> SNAPRRSIHLSNIVEQRVFEDDEIISTPKRGRSKKTVQDNDEDYSPKKSVQKTPTRTRRSSTTTKTATTPSKGITTATATPMTPSQKMKKIRAGELSPSMQQRTDLPAKDSSKSELQLAREQLHVSVVPKSLPCREREFENIYAFLEGKIQDQCGGCMYVSGVPGTGKTATVTGVIRTLQRMAKQNELPAFEYLEINGMRLTEPRQAYVQIYKQLTGKTVSWEQAHALLEKRFTTPAPRRVTTVLLVDELDILCNRRQDVVYNLLDWPTKSAAKLVVVTIANTMDLPERLLMGKVTSRLGLTRLTFQPYSHKQLQEIVTARLGGSETFKGEAVQLVARKVAAVSGDARRALDICRRATEIADTAAVKCVTMLHVQQALAEMIASAKVQAIRNCSRMEQIFLQAIAAEVTRTGVEETTFMGVYQQVETIAAFMGVTFPPPGRALRLCSKLGAERLIISEHSRNDLFQKILLNVSADDIHYALRVEEMVN;> MSASNKGGYKTPRKENLMSIENLTNSEEESEDLNTAMVGNAVESQPKVTSRRSTRRPSPTKKYQAYQKESNGKGQEERIVVNYVEMSDERSSDAEDQEEEESIEESENAARPAAKDLHLIQSEYNVAGTSMFGFNTPKKRDAMALAALNATPCTPKTPKTPRLGVKTPDTKRKKSMDQPKTPAHVRTRVKKQIAKIVADSDEDFSGDESDFRPSDEESSSSSSSSDAGNSSDNDAADDEPKTPSRARRAIVVPVLPKTPSAARLRQSARAKKSNEFVPESDGYFHSHASSKILTSDHTLDRLKNPRLAADRVFSLLSEIKTSAEHEGSINAIMEEYRSYFPKWMCILNEGFNILLYGLGSKHQLLQSFHREVLHKQTVLVVNGFFPSLTIKDMLDSITSDILDAGISPANPHEAVDMIEEEFALIPETHLFLIVHNLDGAMLRNVKAQAILSRLARIPNIHLLASIDHINTPLLWDQGKLCSFNFSWWDCTTMLPYTNETAFENSLLVQNSGELALSSMRSVFSSLTTNSRGIYMLIVKYQLKNKGNATYQGMPFRDLYSSCREAFLVSSDLALRAQLTEFLDHKLVKSKRSVDGSEQLTIPIDGALLQQFLEEQEKK;> MDPTISVSKGCFVYKNGATRAGKKAASKRKRPAAESSSLLGKEVVQQPFYEEYRKAWNQINDHIADLQHRSYARTLEQLVDFVVGQAERDTPDEVLPTAALLTGINQPDHLSQFTALTQRLHAQRAAMVCVLQSRDCATLKAAVETLVFGLVEDNAEVEQMEDEDEDEDGAERDRKRLRRSQCTMKQLKSWYTNNFDSEQKRRQLVVILPDFECFNASVLQDLILILSAHCGSLPFVLVLGVATAMTAVHGTLPYHVSSKIRLRVFQTQAAPTGLNEVLDKVLLSPKYAFHLSGKTFKFLTHIFLYYDFSIHGFIQGFKYCLMEHFFGGNAFALCTDYSKALGRIKQLTHEDMETIRRLPSFRPYVEQINDCKRIIAVLTDDDYLKKKLPQLLRDCLLHFLLFRCSLEFLTELVGDLPRCPLGKLRRELYVNCLNRAIISTPEYKECLQMLSFLSKDEFVAKVNRALERTEQFLVEEIAPLELGEACTAVLRPKLEAIRLAVDEVVKATMATITTTSPNETRQATDHLTPVASRQELKDQLLQRSKEDKMRHQLNTPTTQFGRALQKTLQLIETQIVQDHLRALQDAPPIHELFVFSDIATVRRNIIGAPRAALHTALNNPHFYMQCKCCELQDQSLLVGTLPDLSVVYKLHLECGRMINLFDWLQAFRSVVSDSDHEEVAQEQIDPQIQARFTRAVAELQFLGYIKMSKRKTDHATRLTW;> SNAMPEADRELVSIRRFLKERLQRDYTTLRGYAKERSNVRLLLQRTAEMGESNSLLLLGPRGSGKTTLINSVLADLLPNKSFGENTLIVHLDGNLHTDDRVALKSITVQMQLENAADGKVFGSFAENLAFLLQCLKAGGKHSKSVIFILEEFDLFCAHHNQTLLYNLFDVSQSAQAPICVLGVTCRLDVIELLEKRVKSRFSHRQVFLFPSLRRFEDYVDLCRDLLSLPTGNSLLLAAEKIYNLQNIQSGALYFSRNHFDPGEYGFSPRLRDAWNKQICKVLATQQARSTLQALHDFDISEAYLKNFLFRLVAHLRPQSPHITAEKMAAVGSQFEGDDKIELLCGLSVLELCLIIAIKHHSQIYDRDSFNFEIIYARFSKFAKVSTTMQAVERSIVLKAFEHLRIAELIMPLTGGAGGGVGKVQKEFEMHKLALTYSQIHHCMQRYQALPTEVAQWAQSSLI;> MEAICSSLEPLFPCREAAIETLGELIGDSSETYPSAIYLFGHSGTGKTALTRAFLKECGKRQNVRTAHLNAIECYTTKIMLEILLDSLAPDQGDALKVDNMLDFVEQLRRQAATRVEDQGFLIAVDNAERLRDMDANVLPVLLRLQELTNLNLCVILLSQLPFEKFYNKTGLSEIVCLHLAQYNKAETQRILGSDFQQVRNQLLEQFAQDKKRLEICQEAVTEDFYNNYLNLFLSVFYKACRDVPELQLTARKCLSTYLEPVLDGTVDATDISRLWRHIAGPLRSALTQIYMRIEKPAEEVEDFTAIEDQSVRKLAQSLELPYYAKFLLIAAFLASHNAAKQDKRLFVKHHGKQRKRMQTVNARAKTTEKMSTTLGPKSFSIDRLLAIFYAILEEKVGLTCNLLSQISTLVHLNLLSFVSGEQNIMEGSARLQCTIGLEFVLQIGKVVGFNVRQYLCDFM;> MTTLIEQLITKMGLREEPNVLEKTTELVRLLELRSTNVPLQINEYGKIVLCADLASCMIGIAFDKEQALKLSGLRKSQYLNNKRMFEKLLDLNKLASVNDICVQLGLNEVARKAEELMTLFKGVAATEDMGTDTSHPQYATMAVFQACRLLKKKVSKSKLMPFSNLRPSQFQLLEQQWERMIAKHHKESKVPSSTDMEGKLKENQNENIKGHEAKKAHKPPPED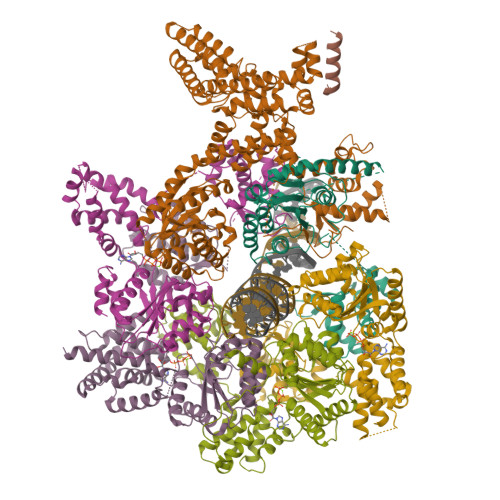YEIWKARMLAKAQAKLKELEASQSHMDSQLLEA;> SNANNLPSPSRNKYQNARRVLNSAETQNLPGRESQLQELREFFSNHLESQTSGSLYVSGQPGTGKTACLSLLLRDPDFSKRLQRVYINCTSIASVGAVYKKLCTELQLKVSGRTERDHLEAIQRHLKTAKRMLLLVLDEIDQLCTSRQEVLYTIFEWPALPGSRILLVGIANSLDLTDRALMRLNARCELKPRLMHFPPYSKQQIVEIFKSRLAEAEVLDVFPPVTLQLLAAKVSAISGDVRRALDIGRRVVEIAEQQKRDGEKEFNMKALQLEGKDAVEAKEKQDTLKPVQVTQVAAVLNKVYGASQNLEEDIEASFPLQQKLMLCTLVLMLRNERNKDISMGRLHEVYRRVCAKRNILALDQAEFTGTVDLVETRGILRIMRKKEPRLHKVLLQWDEEEVHAALSDKQLIASILSDTACLSK> ATVKSVKGFYSFSCN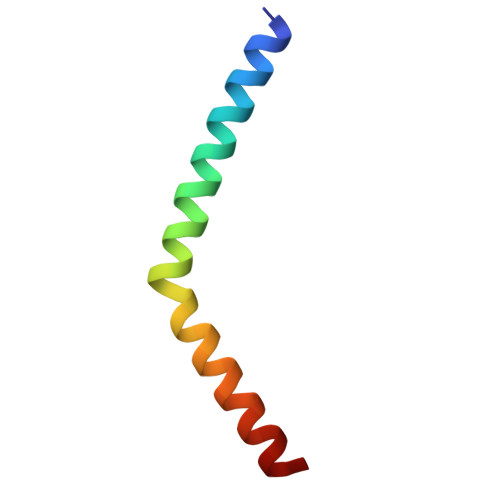ASWIFFTSAVILFAPVIFETERAQMEELHKSQ> GKRERELTMVFESFGFKHGIPIDADYVFDVRFLPNPHW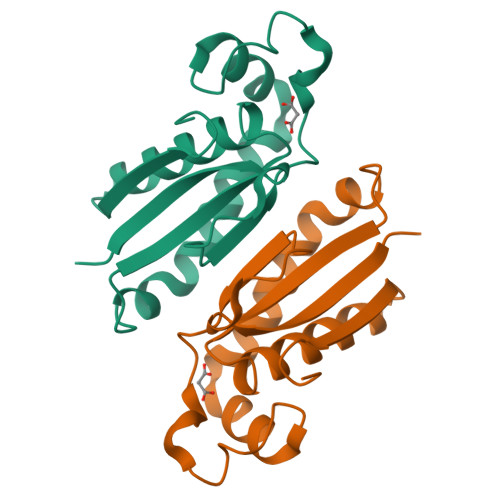DPKLRPMTGLDKPVAAFLDRHTEVHNFIYQTRSYLELWLPMLETNNRSYLTVAIGCTGGKHRSVYIAEQLADYFRSRGKNVQSRHRTLEKRKP>QGMQYEWRKAELIGQLLNLGVTPGGVLLVHSSFRSVRPLEDGPLGLIEALRAALGPGGTLVMPSWSGLDDEPFDPATSPVTPDLGVVSDTFWRLPNVKRSAHPFAFAAAGPQAEQIISDPLPLPPHSPASPVARVHELDGQVLLLGVGHDANTTLHLAELMAKVPYGVPRHCTILQDGKLVRVDYLENDHCCERFALADRWLKEKSLQKEGPVGHAFARLIRSRDIVATALGQLGRDPLIFLHPPEAGCEECDAARQSIG[2x]

Here, we conduct a comprehensive functional analysis of the Antibiotic_NAT family of aminoglycoside acetyltransferases. AG resistance is primarily conferred by three classes of aminoglycoside-modifying enzymes (AMEs): phosphotransferases (APHs), nucleotidylyltransferases (ANTs), and acetyltransferases (AACs). AMEs permanently alter the AG substrate, preventing them from binding to their target, the A-site of the 16S rRNA in the bacterial ribosome. The fold typical of the Antibiotic_NAT family is evident in all structures, composed of 13 α-helices and 8 β-strands, and determined structures superpose with pairwise RMSD’s 0.8–1.0 Å between 197 to 266 matching Cα atoms.

Our structural data includes the crystal structure of the AAC(3)-IVa enzyme which is the first molecular image of a Group 1 Antibiotic_NAT enzyme. Our extensive structural and functional characterization demonstrates that this enzyme mediates broad-spectrum AG resistance, including to 4,5-, 4,6-disubstituted AGs and the atypical AG apramycin by evolving a more spacious active site. This is achieved by a C-terminal extension and modifications of the structure and residue composition of the α4-α5 hairpin of the minor subdomain of the enzyme which allows for broad spectrum of AG recognition. Finally, insert 4 is a C-terminal extension to the major subdomain unique to AAC(3)-IVa and forms an α-helix and a C3H1 Zn2+ binding site. We identified a Zn2+ ion binding site in the C-terminal extension of AAC(3)-IVa structure. This feature may be of only structural significance since neither this ion nor the sidechains of its cysteine and histidine ligands formed any interactions with the AGs. The binding of Zn2+ could stabilize this region and allow for orientation of the Glu249 residue for AG recognition. The Zn2+-binding residues are fully conserved across Antibiotic_NAT Group 1 representatives. The buried surface area between subunits of the AAC(3)-IVa dimer (~650 Å2) was formed nearly exclusively through interactions between the major subdomains of the two monomers of this enzyme. Collectively, these observations show that AGs can adopt multiple bound orientations facilitated by the dramatic structural changes in the minor subdomain of AAC(3)-IVa, thereby supporting broad substrate specificity for AG modification.> IPVIEPLFTKVTEDIPGAEGPVFDKNGDFYIVAPEVEVNGKPAGEILRIDLKTGKKTVICKPEVNGYGGIPAGCQCDRDANQLFVADMRLGLLVVQTDGTFEEIAKKDSEGRRMQGCNDCAFDYEGNLWITAPAGEVAPADYTRSMQEKFGSIYCFTTDGQMIQVDTAFQFPNGIAVRHMNDGRPYQLIVAETPTKKLWSYDIKGPAKIENKKVWGHIPGTHEGGADGMDFDED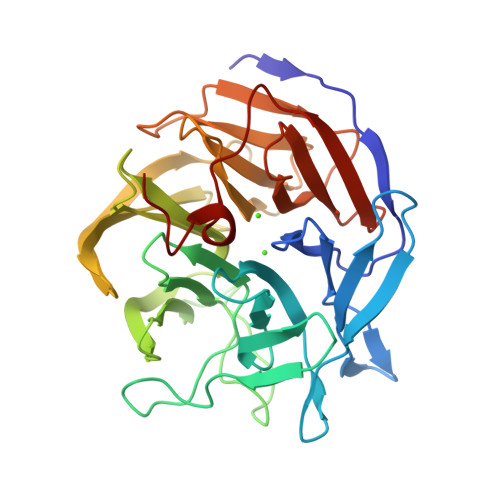NNLLVANLGSSHIEVFGPDGGQPKMRIRCPFEKPSNLHFKPQTKTIFVTEHENNAVWKFEWQRNGKKQYCETLKFGIF> MVSVIDKLVFDFGGKTLVSLAPDNNTLCVANKNGLTKILKTNNPEEEPETLDSSKLVSSIKCYSNSHFLMTTMQGDALRYNIDSSQEELLARFALPLRDCCVIHSGKMAVFGGDDLELILLELDDETHKKHAIKIDEQVSQISYNSQMNILAVSMINGKVQIFSLTSTIPNKVHELNDYIVANSYDDTHRDKILSNMMDDIDKDNDNDLSETADPDENNVADPEFCAANRICTRVAWHPKGLHFALPCADDTVKIFSIKGYSLQKTLSTNLSSTKAHFIDLQFDPLRGTYIAAVDLNNKLTVWNWETSEIHYTREFKRKITNIAWKIQADSKTLDLVLGTWSGSIAIVQNLAESVVSNI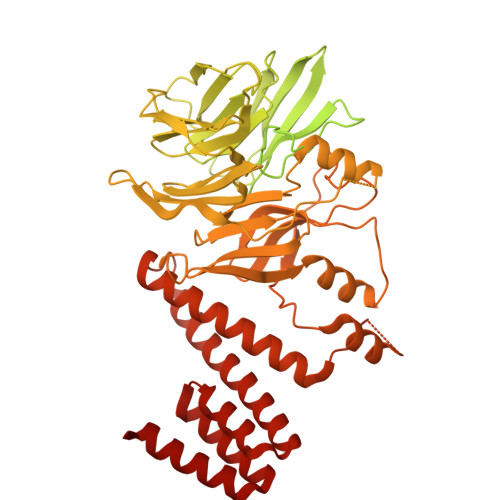PDQSVAESSTKHGLFVDSESDLENLEGNDDINKSDKLFSDITQEANAEDVFTQTHDGPSGLSEKRKYNFEDEEDFIDDDDGAGYISGKKPHNEHSYSRVHKTHSFPISLANTGKFRYMPFSPAGTPFGFTDRRYLTMNEVGYVSTVKNSEQYSITVSFFDVGRFREYHFEDLFGYDLCFLNEKGTLFGQSKTGQIQYRPHDSIHSNWTKIIPLQAGERITSVAATPVRVIVGTSLGYFRSFNQFGVPFAVEKTSPIVALTAQNYRVFSVHYSQFHGLSYSLSELGTSSKRYYKRECPLPMSLPNINSDMKKDANLDYYNFNPMGIKSLFFSSYGDPCIFGSDNTLLLLSKWRSPEESKWLPILDSNMEIWKMSGGKETTDIHVWPLALAYDTLNCILVKGKHIWPEFPLPLPSEMEIRMPVFVKSKLLEENKAILNKKNEIGADTEAEEGEEDKEIQIPVSMAAEEEYLRSKVLSELLTDTLENDGEMYGNENEVLAALNGAYDKALLRLFASACSDQNVEKALSLAHELKQDRALTAAVKISERAELPSLVKKINNIREARYEQQLK D-GLUTAMIC ACID | C5 H9 N O4 | 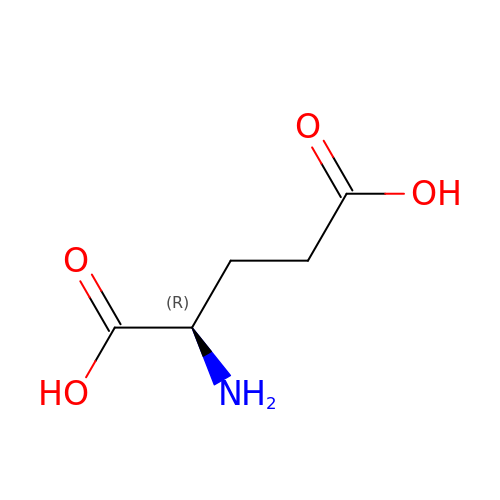WHUUTDBJXJRKMK-GSVOUGTGSA-N> NKVLHQDLVQATRRILKLGPSELRVTDAGLICKNPNYSVCDAMLKTDTVY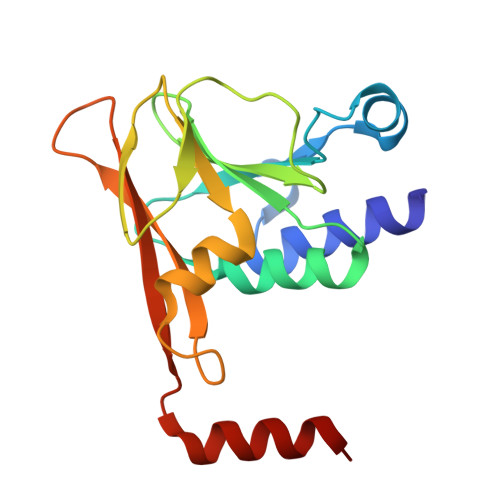CVEYLLSYWESRADHVPCFIFKNTGCAVSLCCFVRAPVALVSPARHVGEFNVLKVNESLIVTLKDIEEIKPSAYGVLTKCVVRKSNSASVFNIELIAFGPENEGEYENLLRELYA1-[(4R)-1,3-oxazolidin-4-yl]methanamine | C4 H10 N2 O | 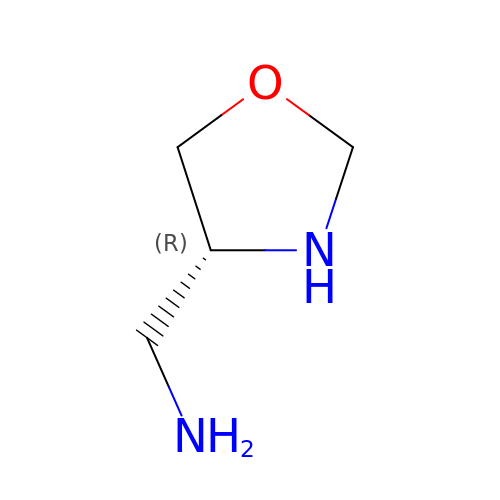JUAFUPTWZIUUQO-SCSAIBSYSA-N>GAHMSGRSSEEVILKDCSVPNPSWNKDLRLLFDQFMKKCEDGSWKRLPSYKRTPTEWIQDFKTHFLDPKLMKEEQMSQAQLFTRSFDDGL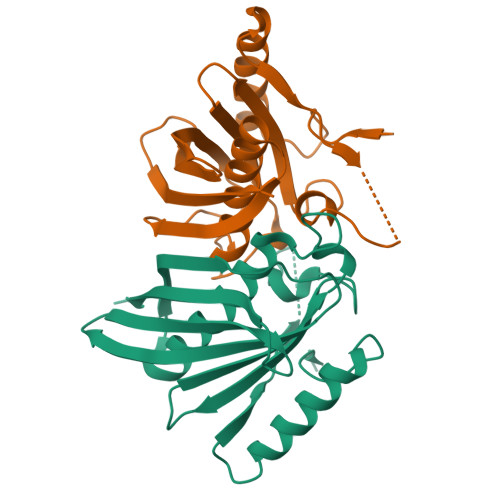GFEYVMFYNDIEKRMVCLFQGGPYLEGPPGFIHGGAIATMIDATVGMCAMMAGGIVMTANLNINYKRPIPLCSVVMINSQLDKVEGRKFFVSCNVQSVDEKTLYSEATSLFIKLNPAKSLT[4x]(6R,7S,10Z)-10-(2-amino-1,3-thiazol-4-yl)-1-(1,5-dihydroxy-4-oxo-1,4-dihydropyridin-2-yl)-7-formyl-13,13-dimethyl-3,9-dioxo-6-(sulfoamino)-12-oxa-2,4,8,11-tetraazatetradec-10-en-14-oic 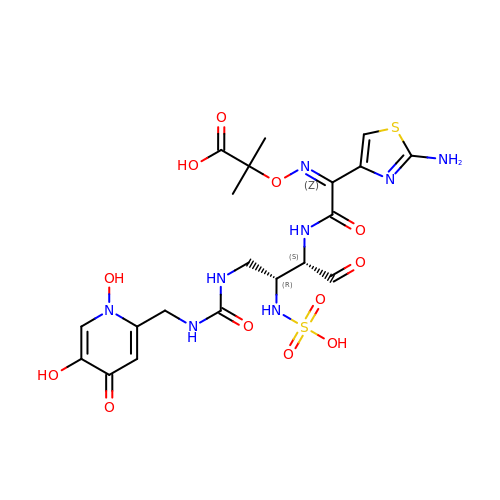acid | C20 H26 N8 O12 S2 | DRGQACYRFXBYPT-SATPWBBZSA-N> MAQILPIRFQEHLQLQNLGINPANIGFSTLTMESDKFICIREKVGEQAQVVIIDMNDPSNPIRRPISADSAIMNPASKVIALKAGKTLQIFNIEMKSKMKAHTMTDDVTFWKWISLNTVALVTDNAVYHWSMEGESQPVKMFDRHSSLAGCQIINYRTDAKQKWLLLTGISAQQNRVVGAMQLYSVDRKVSQPIEGHAASFAQFKMEGNAEESTLFCFAVRGQAGGKLHIIEVGTPPTGNQPFPKKAVDVFFPPEAQNDFPVAMQISEKHDVVFLITKYGYIHLYDLETGTCIYMNRISGETIFVTAPHEATAGIIGVNRKGQVLSVCVEEENIIPYITNVLQNPDLALRMAV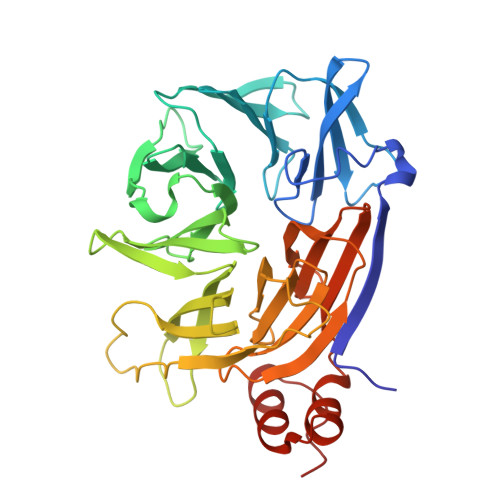RNNLAGAEELF>[3x]MTNIAKAQPKLYVMDNGRMRMDKNWMIAMHNPATIANPNAPTEFIEFPIYTVLIDHPEGKILFDTSCNPDSMGAQGRWGEATQSMFPWTASEECYLHNRLEQLKVRPEDIKFVIASHLHLDHAGCLEMFTNATIIVHEDEFSGALQTYARNQTEGAYIWGDIDAWIKNNLNWRTIKRDEDNIVLAEGIKILNFGSGHAWGMLGLHVQLPEKGGIILASDAVYSAESYGPPIKPPGIIYDSLGFVRSVEKIKRIAKETNSEVWFGHDSEQFKRFRKSTEGYYE

AaL (WP_021296945.1) is a lactonase isolated from the acidophilic, moderately thermostable bacterium Alicyclobacillus acidoterrestris. The quorum quenching lactonase AaL from the thermoacidophilic bacterium Alicyclobacillus acidoterrestris exhibits a very broad substrate range, being capable of hydrolyzing short and long chain AHLs with high proficiencies. AaL possesses a bi-metallic active site center. We show that AaL is capable of degrading δ-lactones and γ-lactones with high catalytic proficiency (>104 M−1 s−1) and shows some weak, promiscuous phosphotriesterase activity on the insecticide-derivated paraoxon. The crystal structure of AaL reveals a unique hydrophobic patch which could relate to its high specificity, and highlights a flexible active site loop which may be involved in substrate binding.

AaL was also crystallized bound to a glycerol molecule. Glycerol may originate from the cryoprotectant solution that contains glycerol. The molecule interact through two of its alcohol groups with the metal cations and with D122. In fact, an alcohol group is bridged with the α-metal, D122 and D220 at 2.0, 2.6 and 2.7 Å respectively and the second alcohol interacts with the β-metal (1.9 Å). Surprisingly, whereas the metal coordination is very similar to other lactonases from the MLL family (AiiA, AiiB, AidC) and the PLL family (SsoPox, SisLac, VmoLac), and the good resolution of the structure (2.15 Å), the putative metal cation-bridging water molecule is not visible in the electronic density maps. It is however difficult to conclude whether this molecule is present or not, since the observation of this water molecule can be difficult because of the strong density peaks corresponding to both metal cations, and the conserved coordination suggests that the conserved bridging water is present in AaL. When compared to the AaL structure bound to phosphate, both structures align very well, with the exception of the 237-loop. Additionally, the metal coordination is slightly different in the two structures. Indeed, the distance between the two metal cations is bigger in the glycerol bound structure, as compared to the phosphate bound one (4.0 Å and 3.5 Å, respectively). This lead to a shift in the position of the residues H120, H123, H266 and D220 which coordinates the metals.>[6x]GSDIGQVIHPDDFDKAAADDYVLHEDGE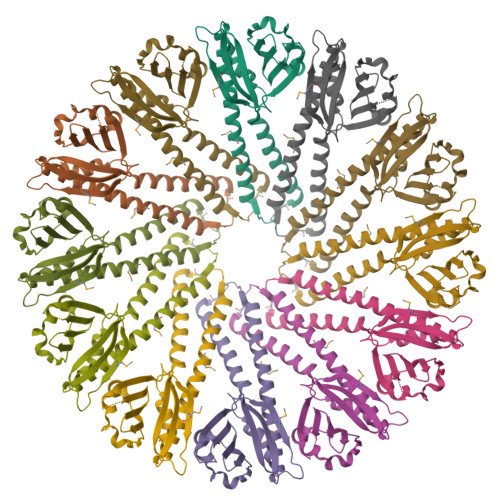KIYFLIKSKTDEYCFTNLALVHLDGESAVSSKRVLYRYPYAHYPIRHVMFETAGTVDLDVEIKFEIGGKHYSIDVDKKQLEHVKDLYKALLAIAEKQYEGQKMLEFANSSLNHSVTILGGLRQGDMNVPQTFKDLSQESFDWLQGHYYKWNQKDFGSFYEKYINN>[2x]MSSVTWAPGNYPSTRRSDHVDTYQSASKGEVPVPDPYQWLEESTDEVDKWTTAQADLAQSYLDQNADIQKLAEKFRASRNYAKFSAPTLLDDGHWYWFYNRGLQSQSVLYRSKEPALPDFSKGDDNVGDVFFDPNVLAADGSAGMVLCKFSPDGKFFAYAVSHLGGDYSTIYVRSTSSPLSQASVAQGVDGRLSDEVKWFKFSTIIWTKDSKGFLYQRYPARERHEGTRSDRNAMMCYHKVGTTQEEDIIVYQDNEHPEWIYGADTSEDGKYLYLYQFKDTSKKNLLWVAELDEDGVKSGIHWRKVVNEYAADYNIITNHGSLVYIKTNLNAPQYKVITIDLSKDEPEIRDFIPEEKDAKLAQVNCANEEYFVAIYKRNVKDEIYLYSKAGVQLTRLAPDFVGAASIANRQKQTHFFLTLSGFNTPGTIARYDFTAPETQRFSILRTTKVNELDPDDFESTQVWYESKDGTKIPMFIVRHKSTKFDGTAAAIQYGYGGFATSADPFFSPIILTFLQTYGAIFAVPSIRGGGEFGEEWHKGGRRETKVNTFDDFIAAAQFLVKNKYAAPGKVAINGASNGGLLVMGSIVRAPEGTFGAAVPEGGVADLLKFHKFTGGQAWISEYGNPSIPEEFDYIYPLSPVHNVRTDKVMPATLITVNIGAGRVVPMHSFKFIATLQHNVPQNPHPLLIKIDKSWLGHGMGKPTDKNVKDAADKWGFIARALGLELKTVE;>[2x]IWGIGCNPWTAEHVDQTLASGNDIC

GmPOPB is the macrocyclase responsible for macrocyclization of amatoxins, eight amino-acid ribosomal peptides with the core sequence IWGIGC(N/D)P. Amatoxins are cyclic peptides further modified by a characteristic sulfoxide cross-link between tryptophan and a cysteine, and hydroxylation (the extent of which vary). GmPOPB is an unusual enzyme catalyzing, depending on substrate length, proteolysis, or macrocyclization using the same catalytic machinery. The protein contains two domains as observed in other POP enzymes. The domain containing the putative catalytic residues (Ser577, Asp661, His698) comprises residues 1–81 and 450–728, and the other domain is a seven bladed β-propeller, comprising residues 82–449.

In order to obtain co-complexes, we mutated each residue of the presumed catalytic triad (mutants S577A, D661A, and H698A) to ensure inactive protein. Crystals were obtained for the 35mer complex for S577A and H698A; with the 25mer substrate S577A and D661A. In all 35mer and 25mer complexes, the enzyme adopts the same “closed” conformation in which the lid (the propeller domain) sits on top of the catalytic domain. In both 25mer complexes the N-terminal residues of the substrate (IWGIGCN) are disordered; in the S577A–35mer complex the N-terminal two residues (MF) are missing, while in the H698A complex only the first N-terminal residue is absent. There are also no major differences between the H698A–35mer and S577A–35mer complexes, and between the S577A–25mer and D661A–25mer complexes. The oxyanion-stabilizing Tyr496 is in close proximity to the core proline (P8) in the 25mer structure (D661A mutant), while Tyr496 hydrogen bonds with P18 in the 35mer complex. Substrate residues I11–P18 (the core peptide is not seen in the 25mer, apart from weak density from P8 in the D661A–25mer complex) form a twisted loop, which makes contacts with the protein and within itself; atoms that will ultimately form the macrocycle are 7.6 Å apart. To confirm the importance of the putative catalytic triad for GmPOPB, the mutants S577A, D661A, and H698A were evaluated for activity, and were inactive with both 25mer and 35mer substrates, using 5 μM GmPOPB and monitoring the reaction progress after 24 h. The recognition tail adopts an identical distorted 310 helix conformation inserted into the middle of the β-propeller domain in both the 25mer and 35mer complexes.>EHAERLPYDASKWEFPRDRLKLGKPLGRGAFGQVIEADAFGIDKTATCRTVAVKMLKEGATHSEHRALMSELKILIHIGHHLNVVNLLGACTKPGGPLMVIVEFCKFGNLSTYLRSKRNEFVPYKVAPEDLYKDFLT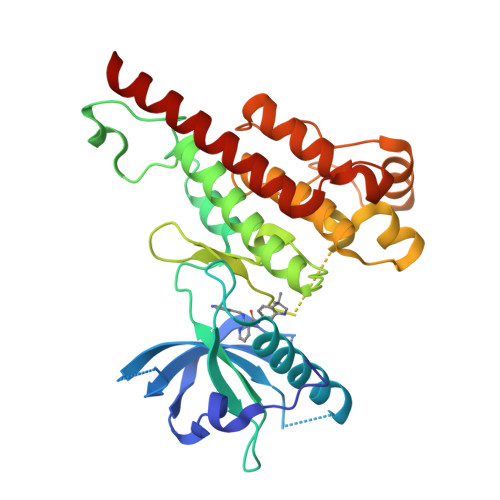LEHLICYSFQVAKGMEFLASRKCIHRDLAARNILLSEKNVVKICDFGLARDIYKDPDYVRKGDARLPLKWMAPETIFDRVYTIQSDVWSFGVLLWEIFSLGASPYPGVKIDEEFCRRLKEGTRMRAPDYTTPEMYQTMLDCWHGEPSQRPTFSELVEHLGNLLQANAQQDRHHHHHH[2x]BIS(((3S,4S,5R,6R)-5-(ETHYL(PHOSPHORYLOXY))-3,4,6-TRIHYDROXY-TETRAHYDRO-2H-PYRAN-2-YL)METHYL) HYDROGEN PHOSPHATE | C16 H33 O20 P3 | 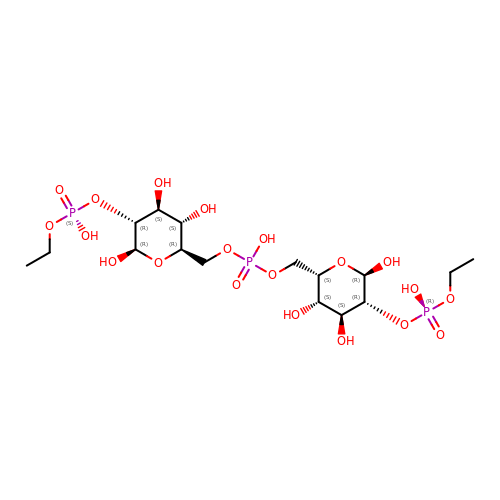QTCHWELPTUAUQX-ASCZGESISA-N> MAEKSIFNEPDVDFHLKLNQQLFHIPYELLSKRIKHTQAVINKETKSLHEHTAALNQIFEHNDVEHDELALAKITEMIRKVDHIERFLNTQIKSYCQILNRIKKRLEFFHELKDIKSQNSGTSHNGNNEGTRTKLIQWYQSYTNILIGDYLTRNNPIKYNSETKDHWNSGVVFLKQSQLDDLIDYDVLLEANRISTSLLH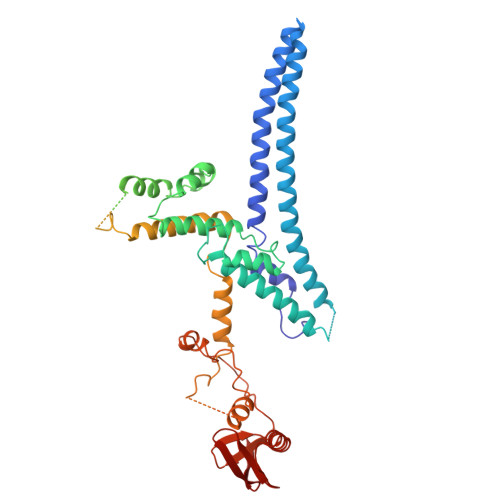ERNLLPLISWINENKKTLTKKSSILEFQARLQEYIELLKVDNYTDAIVCFQRFLLPFVKSNFTDLKLASGLLIFIKYCNDQKPTSSTSSGFDTEEIKSQSLPMKKDRIFQHFFHKSLPRITSKPAVNTTDYDKSSLINLQSGDFERYLNLLDDQRWSVLNDLFLSDFYSMYGISQNDPLLIYLSLGISSLKTRDCLHPSDDENGNQETETATTAEKEVEDLQLFTLHSLKRKNCPVCSETFKPITQALPFAHHIQSQLFENPILLPNGNVYDSKKLKKLAKTLKKQNLISLNPGQIMDPVDMKIFCESDSIKMYPT> MRGSHHHHHHGSRGSEVGPALFQSDMTFKIFIDGEVNGQKFTIVADGSSKFPHGDFNVHAVCETGKLPMSWKPICHLIQWGEPFFARYPDGISHFAQECFPEGLSIDRTVR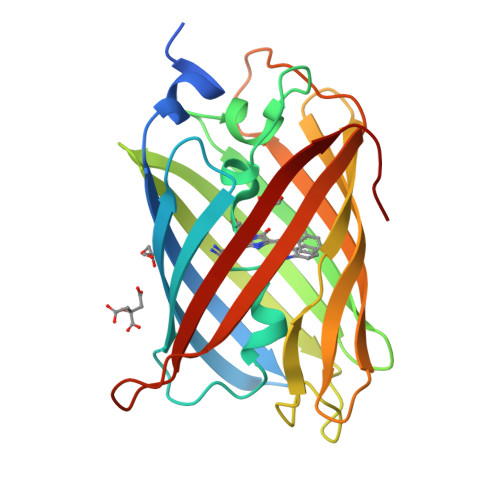FENDGTMTSHHTYELDDTCVVSRITVNCDGFQPDGPIMRDQLVDILPSETHMFPHGPNAVRQTATIGFTTADGGKMMGHFDSKMTFNGSRAIEIPGPHFVTIITKQTRDTSDKRDHVCQREVAYAHSVPRI S-Thalidomide | C13 H10 N2 O4 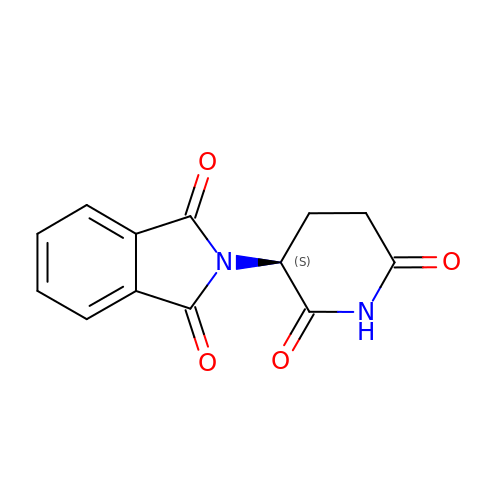| UEJJHQNACJXSKW-VIFPVBQESA-N P. aeruginosa encodes three distinct T6SS hemolysin coregulated protein (Hcp) secretion islands (named H1-to H3-T6SS) that act against both prokaryotic and eukaryotic cells. TplE, a novel H2-T6SS-dependent lipase effector, was recently identified. TplE is an antibacterial lipolytic toxin and TplEi interacts with TplE to provide protection from TplE. TplE, a new T6SS trans-kingdom toxin, targets the conserved and essential cell membranes of rival bacteria to cause bacteriolysis, while TplEi functions as a cognate immunity protein to prevent self-intoxication.

Herein, we solved the crystal structure of TplEi in complex with a TplE peptide (residues 82-108) generated by treatment with subtilisin. As anticipated, after 30 days of proteolysis and crystallization, we first observed crystals growing from the subtilisin-treated TplE-TplEi complex sample, and crystals diffracted the X rays to 2.2Å. Surprisingly, the majority of TplEi was intact, whereas TplE had been degraded except for a 27 residue fragment that remained bound to TplEi. Residues 82-108 of TplE is comprised α1 and α2 helices that are connected by a disordered loop region. Because α1 is significantly longer than α2 and the two helices are nearly perpendicular to each other, the peptide exhibits a “L” shape, thus, we designated it as “L” peptide based on its shape. The “L” peptide accommodates a negatively charged groove of domain II of TplEi. Details of the TplE “L” peptide interaction with TplEi involves two salt bridges, eight hydrogen bonds and 147 non-bonded contacts through PDBsum analysis. In particular, “L” peptide residue K100 is anchored in the deep pocket through four hydrogen bonds formed with TplEi residues S215, T216, and G217. The structural superimposition of the “L” peptide and TplE aligned 25 Cα atoms with a rmsd value of 0.59Å, indicating that the conformation of the “L” peptide alone is nearly identical to its conformation in the context of the full protein. The TplE peptide (denoted the “L” peptide) has a high binding affinity for TplEi in vitro and precludes the formation of the TplE-TplEi complex, which in turn releases the toxicity of TplE and thereby induces bacterial cell death.

> MGSSHHHHHHSSGLVPRGSHMSSSRSSSMDKTGWITHCFGRFLIDLPPDAVINAGYYLWGDRIEYLDDKPTELAARVDRLEQEWRTQRHKSKGNMFLRKIDFGNESVGLLSWSSEVASKTYLLDTYVTSKPTWHVYRWKGKVSVDREQHAVEISRALARNLRSRAPKEIPSEPGFCIDHAYIAGDSFQVERFGVGVTFPEHPGARFEFRSSTGAELNSLLERVDGFVQNMLSTFAGMETLRKGKHPVGSLPGEEYLVAGSDKGQRGYTFMWEVQGKEESLTEPNLTAGLAVLERSNENGKPPPPAFKSDKEALELWDTIVDSIRVRPTSSSPRGGNAGPSPAPKPATPGGQTLGDHYVYEEFLSSLKPKDSWLDDL;> DDLFASIGALWTWAWRGPKARQELLKA> STITSSLDVRPEIKQAVTVRPGMCGPGSLFVGQLGDWTWETVSAQCDTDVFAARDASGNPTYLAFYYFRVRGGRELHPGSLTFGDRLTVTSGCYDQ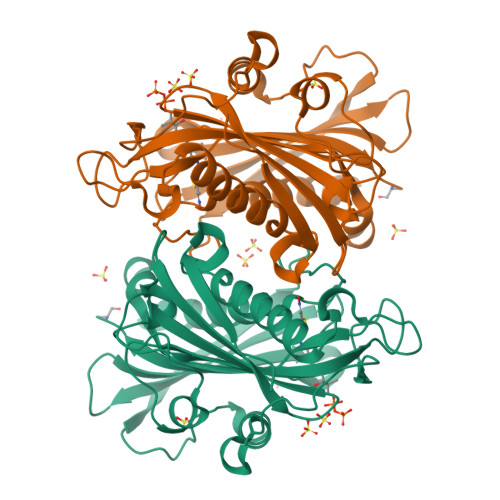GTESVLTLHRIDRAGSDDAQRPLDLHEFYERPRDGSLYVENFNRWVTRSAPGSNEDLVKSSPPGFRNDGLPQLPAAYSPRAVYREARTAHTFRALDEPGFRLLPDTVEVEHPVDIVRDVNGVGLLYFASYFSMVDKAALALWRRLGRSDRAFLRRVVVDQQMCYLGNADLDSVLTLGARVRVSTETPGEELVDVVISDRDSGRVIAVSTLHTQHDAHDPKGEA>GQDLALSCGTSEASADQDKKKWEPDTKFLKTGNSIHATATYQDPSLLSTVPYMTARIFTAPATYEIPIKGDKRHLLRLYFYPSTYTGLNISNSYFTVEANDVTLLSNFSAAITCQALTQAYLVKEYSLAPTDKDVLSIKFTPSDKYRDAFAFINGIEVIQMPELFDTAALVGFTDQTMDAKTANLQSMFRLNVGGQDIPGSQDSGGLTRTWYNDAPYIFSAGLGVTLQASNNFRINYQNMPVSIAPADIYKTARSQGPNGDINLKSNLTWMFQIDKNFTYILRLHFCEFQLSKINQKVFNIYINNRTAQADTTPADIIGWTGEKGIPMYKDYAIYVDANNGGEEITLQMTPSTFGQPEYYDSSLNGLEIFKMDTMKNLAGPNPEP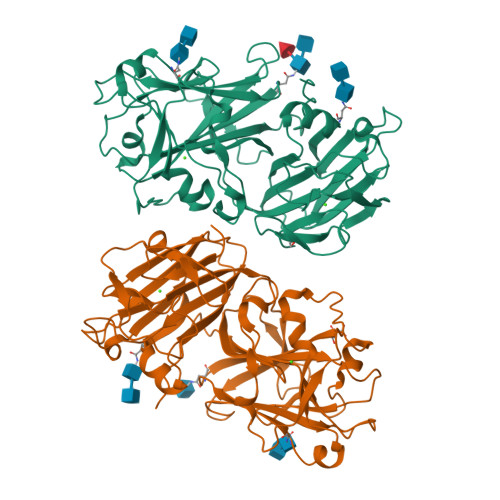SPMQAEEEVKKEFKNEKRHLEGSENLYFQ[2x]>[3x]VPGPEYKVAILTVSDTVSAGAGPDRSGPRAVSVVDSSSEKLGGAKV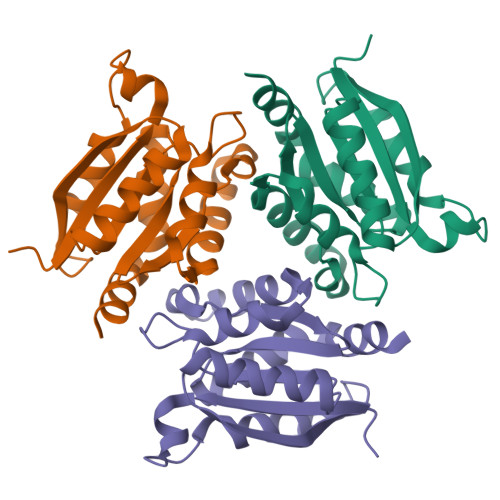VATAVVPDEVERIKDILQKWSDVDEMDLILTLGGAGFTPRDVTPEATKKVIERETPGLLFVMMQESLKITPFAMLSRSAAGIRGSTLIINMPGNPNAVAECMEALLPALKHALKQIKGDKR>[4x]MGHHHHHHMVLMTKPGTSDFVWNGIPLSMELNLWNIKEYSGSVAMKFDGEKITFDADIQNLSPKEPERYVLGYPEFYYGYKPWENHTAEGSKLPVPVSSMKSFSVEVSFDIHHEPSLPLNFAMETWLTREKYQTEASIGDVCIMVWFYFNNLTPGGEKIEEFTIPFVLNGESVEGTWELWLAEWGWDYLAFRLKDPVKKGRVKFDVR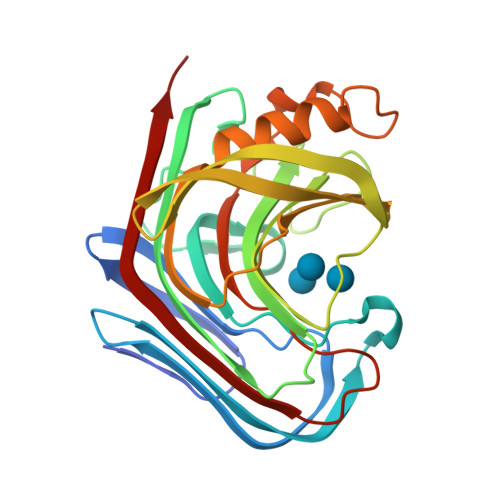HFLDAAGKALSSSARVKDFEDLYFTVWEIGTEFGSPETKSAQFGWKFENFSIDLEVRE> MAFSGSQAPYLSPAVPFSGTIQGGLQDGLQITVNGTVLSSSGTRFAVNFQTGFSGNDIAFHFNPRFEDGGYVVCNTRQNGSWGPEERKTHMPFQKGM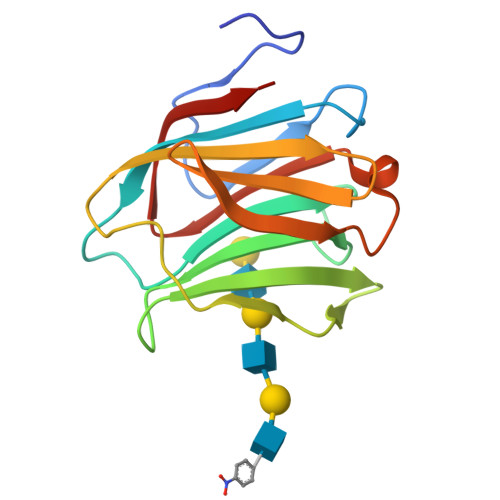PFDLCFLVQSSDFKVMVNGILFVQYFHRVPFHRVDTISVNGSVQLSYISFQ>MVPTQAHPEWYKSAVFYELSVRTFQDGNGDGKGDFPGLTSRLDYLKNLGVDCLWLLPWFPSPLRDDGYDVADYRGIHPDLGTLDDFKVFLREAHARGLWVIGDLVTNHTSSDHPWFQAARRGPTLPDGSPNEYHDYYVWSDEGKEYADTRIIFTDTEVSNWTLDEQAGKYYWHRFFASQPDLNYDNPKVVEELHGAARFWLDLGLDGFRVDAVPYLIEREGTSCENLPETHEILKGFRAMVDREYPGRLLLAEAFQWPEEVVEYFGTEAEPEFHMCFNFPVMPRLYMSLKREDTSSIREIMGRLPKIPSFGQWCIFLRNHDELTLEMVTDDERAFMYAAYAPDARMKINVGIRRRLAPLLDNDRRRIELLNTVLLALPGSPVLYYGDEIGMGDDLGLPDRNGVRTPMQWNAGTSGGFSTAQPSDC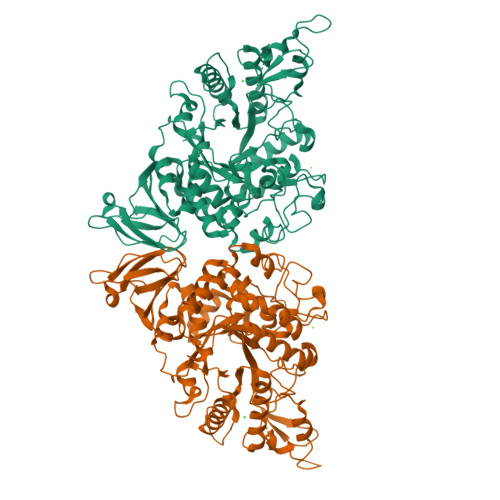FFPPIQDPVYGFGRVNVQSQLQDPSSLLKWTARQLELRRAHPAFAHGDLTFIETGNPAILAFTRQYDGETLLIVSNFAGNAQAGLLDLAPFVGRAPVTLSGASPLPVVTGNGQYPVVMGKYDYYWLRLNSRVDKLAAALEHHHHHH[4x]>GCGGGGACGACCCCGC[4x]

The guanidine-II (mini-ykkC) riboswitch is the smallest of the guanidine-responsive riboswitches, comprising two stem loops of similar sequence. The guanidine riboswitches bind the guanidinium cation such that the level of expression of genes that deal with guanidine toxicity is upregulated. Crystal structures of these stem loops show that they are intrinsically disposed to dimerization by loop-loop interaction. The loop-loop interaction creates binding sites for two guanidine molecules, and thus the folded conformation of the RNA is stabilized by guanidine binding, which leads to the increased level of gene expression.

The crystals are orthorhombic (P212121), and two dimeric RNA complexes comprise the asymmetric unit (ASU). Each dimer within the ASU is created by a close association between the two ACGA terminal loops, with almost coaxial alignment of the two stems. The central C8 and G9 of each loop make complementary cis Watson-Crick base pairs, i.e., cross-strand C8-G9′ and G9-C8′ base pairs. A7 is coplanar with the closing G6′-C11′ base pair from the other stem loop, hydrogen bonding to the sugar edge of C11′, between A7N6-C11′O2 and A7N1-C11′O2′. At the other end of the loop A10 and A10′ nucleobases are extruded and inclined at 20° to the helical axis, and are mutually stacked with a spacing of 3.3 Å. The interacting loops of the dimer together create two binding sites for guanidine molecules. Each guanidine molecule binds coplanar with the G9-C8′ base pair, hydrogen bonded to G9 O6 and N7. The remaining amine of each guanidine is hydrogen bonded to the proS and proR non-bridging oxygen atoms of phosphates of A7 and C8, respectively, at the very tight turn of the loop. The guanidinium cation is stacked upon the nucleobase of G6, making a cation-π interaction (Gallivan and Dougherty, 1999, Wintjens et al., 2000). The space above the guanidine is closed off by the nucleobases of C8 and A7, and thus the ligand is enclosed in a box, except for a space between the backbones of both loops at their tight turns, on the major groove side of the cross-strand C-G base pairs.> ACSFPKCPWVEGCAX;> GPGYQDPLSIDERLQALVYRELNNAVAFNKAESGSAVLVDVNTGEVLAMANSPGRNRTITDVFEPGSTVKPMVVMTALQRGVVRENSVLNTIPYRINGHEIKDVARYSELTLTGVLQKSSNVGVSKLALAMPSSALVDTYSRFGLGKATNLGLVGERSGLYPQKQRWSDIERATFSFGYGLMVTPLQLARVYATIGSYGIYRPLSITKVDPPVPGERVFPESIVRTVVHMMESVALPGGGGVKAAIKGYRIAIKTGTAKKVGPDGRYINKYIAYTAGVAPASQPRFALVVVINDPQAGKYYGGAVSAPVFGAIMGGVLRTMNIEPDALTTGDKNEFVINQGEGTGGRS

Within the family of genes that encode peptidoglycan production the gene product of ftsI, named PBP3 in E. coli, is an essential monofunctional, Class B PBP transpeptidase. PBP3 catalyses the cross-linking of peptide stems from adjacent glycan strands in peptidoglycan to create the strong, mesh-like structure of the final polymer. The β-lactam class of antibiotics, which includes penicillins, cephalosporins, monobactams and carbapenems, exhibit efficacy against both Gram-negative and Gram-positive bacteria and are well tolerated, efficacious and broadly prescribed. Their mechanism of action is through covalently modifying the active site serine in the transpeptidase site of PBPs, leading to the inhibition of cell well biosynthesis and cell death. Bicycle molecules are bicyclic peptides formed through the structural constraint of peptides around a trimeric scaffold via the formation of thioether cysteine linkages.

The Bicycle molecule binds in the active site cleft, in a region previously demonstrated as the binding site for β-lactams such as piperacillin and AIC499, a newer monobactam. The buried surface area of the peptide bound to the protein is approximately double that of the buried surface area of the protein reacted with piperacillin (1832 Å2 and 951 Å2 respectively). Compared to apo structures of EcPBP3, the backbone conformation of the bound EcPBP3 is largely unchanged despite the presence of the large ligand (RMSD of 0.357 Å). The peptide adopts a rough “Figure-of-8” conformation within the active site, with the N- and C-terminus of the peptide linked via two arms of the scaffold and completing the “8”. The peptide is 5.3 Å away and only interacts with the conserved active site catalytic residues (i.e. Ser307, Lys 310, Ser359, Asn361, Lys494 and Thr495) via bridging waters. Loop 1 of the peptide extends beyond the binding footprint of β-lactams within the transpeptidase catalytic site of EcPBP3, with Phe2 binding a previously unengaged pocket of EcPBP3 created by Glu304, Met422 and Val501 of the protein. Trp6 of the peptide interacts with a hydrophobic wall comprising Tyr541, Tyr511 and Lys499 of EcPBP3, in a similar fashion to the interactions of the gem-dimethyl group of aztreonam with Tyr503, Tyr532 and Phe533 of P. aeruginosa PBP331. Val7 participates in intramolecular interactions with the TATA scaffold and C-terminal cysteine, making a significant contribution to the positioning of the C-terminal half of the peptide. The electron density for the peptide residues and the scaffold moiety is largely complete, with the exception of the lysine sidechain and N-terminal residues.>[2x]MVSNGGLLRVGLKK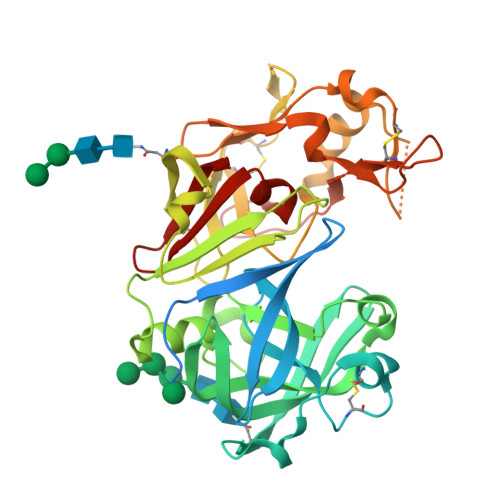RKVDRLDQLRAHGVHMLGNARKDFGFRRTLRDSGSGIVALTNDRDTAYYGEIGIGTPPQNFAVIFDTGSSDLWVPSTKCDTSLACVIHPRYDSGDSSTYKGNGTTASIQYGTGAIVGFYSQDSVEVGDLVVEHQDFIETTEEDDTVFLKSEFDGILGLGFQEISAGKAVPVWYNMVNQGLVEEAVFSFWLNRNVDEEEGGELVFGGVDPNHFRGNHTYVPVTRKGYWQFEMGDVLIGDKSSGFCAGGCAAIADSGTSFFAGPTAIITQINQAIGAKGGGGSAESIVDCNGISSMPNIAFTIGSKLFEVTPEQYIYKVGEGEAATCISGFTALDIMSPQGPIWILGDMFMGPYHTVFDYGKLRVGFAEAV> MSVKASGGSSLARPQLYQTVPVSAISQAEQQDRFLEGSELNELTAYFQSGALRLEIAETLTQNADLIVSRAANRIFTGGSPLSYLEKPVERQPALVGASSDSRNGSVTYAESNGSGGLFGGLRSVFSSTGPIPPGFRPINIARYGPSNMQKSLRDMSWFLRYTTYAIVAGDPNIIVVNTRGLKEVIENACSIDATIVAIQEMRAASADYFRNNAQAKEIVLQYFDIL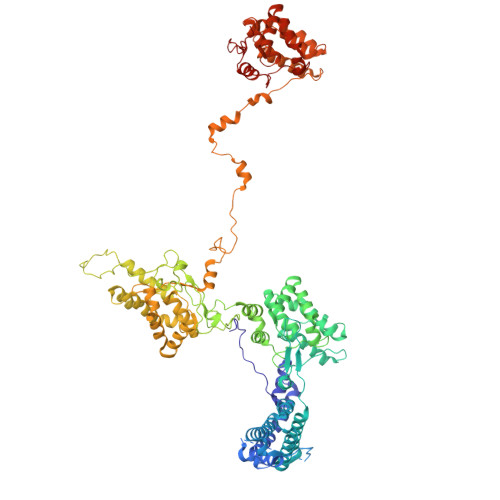LSEFKAPTPANKVRQGPSNDIQGLELPQSYFNAAAKRQKYAMKPGLSALEKNAVIKAAYRQIFERDITKAYSQSISYLESQVRNGDISMKEFVRRLAKSPLYRKQFFEPFINSRALELAFRHILGRGPSSREEVQKYFSIVSSGGLPALVDALVDSQEYADYFGEETVPYLRGLGVEAQECRNWGMQQDLFSYSAPFRKVPQFITTFAQYDRPLPDQHVYGSGNDPLEIQFGAIFPKETRNPSKRPAPFNKDTKRILIHRGPAVNNQVGNPSAVGEFPGSLGAKVFRLNGGLPGAKVGKNTGTSVKFGESSTQALIRAAYRQVFGRDLYEGQRLSVAEIQLENGDISVREFIKRLAKSELFLKLYWAPHYVCKAIEYMHRRLLGRPTYGRQEMNQYFDIASKQGFYAVVEAMIDSKEYSDAFGEDTVPYERYLTPGGLQMRSARVGSLREDIGQRVDKEVTPRFVELGQVSAIRTEPEIAYRSNQGVTRQRQQTKVFKLVSTYDKVAVKNAIRAAYRQVFERDLEPYIINSEFTALESKLSNNEINVKEFIEGLGTSELYMKEFYAPYPNTKVIEMGTKHFLGRAPLNQKEIQQYNQILASQGLKAFIGAMVNGMEYLQTFGEDTVPYRRFPTLPAANFPNTERLYNKLTKQDKELVVPSFTPVVKVGG>MKCTKNALAQTGFNKDKYFNGDVWYVTDYLDLEPDDVPKRYCAALAAGTASGKLKEALYCYDPKTQDTFYDVSELQEESPGKYTANFKKVEKNGNVKVDVTSGNYYTFTVMYADDSSALIHTCLHKGNKDLGDLYAVLNRNKDTNAGDKVKGAVTAASLKFSDFISTKDNKCEY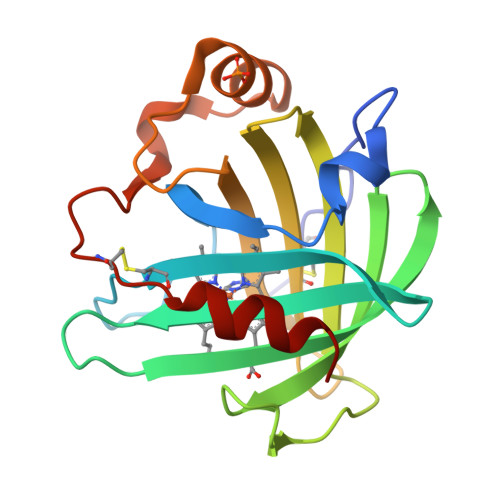DNVSLKSLLTK[2x]> TPGIVIPPQEQITQHGSPYGRCANKTRALTVAELRGSGDLQEYLRHVTRGWSIFALYDGTYLGGEYGGVIKDGTPGGAFDLKTTFCIMTTRNTGQPATDHYYSNVTATRLLSSTNSRLCAVFVRSGQPVIGACTSPYDGKYWSMYSRLRKMLYLIYVAGISVRVHVSKEEQYYD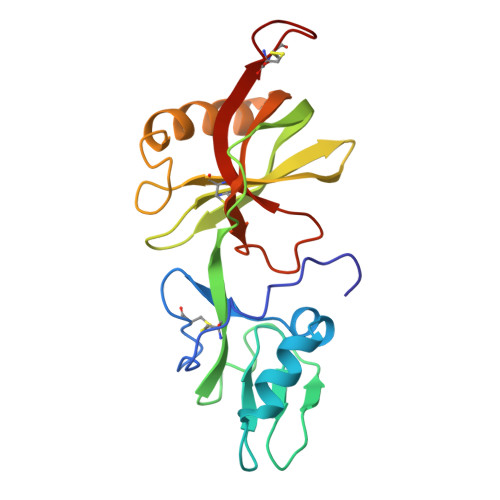YEDATFETYALTGISICNPGSSLC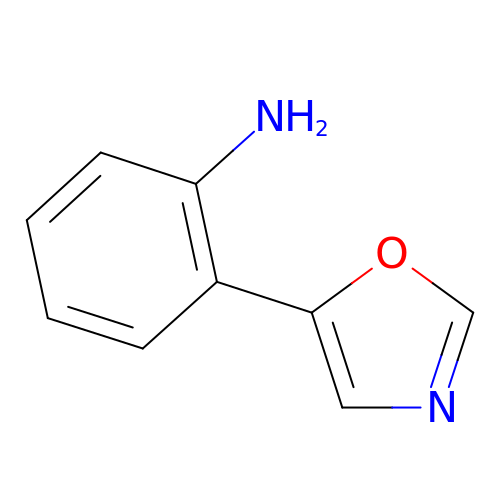2-(1,3-oxazol-5-yl)aniline | C9 H8 N2 O | UZPQWOKKMYUKNI-UHFFFAOYSA-N> GAMGDVSRLNQRNINELKIFVEKAKYYSIKLDAIYNECTGAYNDIMTYSEGTFSDQSKVNQAISIFKKDNKIVNKFKELEKIIEEYKPMFLSKLIDDFAIELDQAVDNDVSNARHVADSYKKLRKSVVLAYIESFDVISSKFVDSKFVEASKKFVNKAKEFVEENDLIALECIVKTIGDMVNDREINSRSRANNFAKKEADFLGAAVELEGAYKAIKQTLL

Lyme borreliae produce other outer surface proteins, including CspZ (also known as BbCRASP-228,29). CspZ promotes bacterial dissemination to distal tissues by evading the complement system, the first-line innate immune defense in vertebrates in the blood, through binding and recruiting a host complement inhibitor, factor H (FH). Additionally, CspZ is only produced after Lyme borreliae invade vertebrate hosts and, as such, induces CspZ-specific immune responses after natural infection. Similar to CspZ, CspZ-YA is an all-α-helical protein composed of nine α-helices (denoted as helices A to I).

Here, we solve the crystal structure of a mutated Bb vaccine antigen, CspZ-YA that lacks the ability to bind to host complement factor H (FH). However, in CspZ-YA, the distance fluctuates between 2.6 and 31.8 Å but mostly greater than 4 Å. Such a distance is unfavorable for the formation of the salt bridge, suggesting the destabilization of CspZ-YA. Additionally, the three-dimensional structure of CspZ revealed a hydrophobic core between helices G, H and I where residues Y207 and Y211 are on one side, along with F176, I183 and F217 on the other side. Unlike CspZ, a cavity was found in CspZ-YA due to the replacement of two bulky and non-polar amino acid residues, Y207 and Y211, with alanine (the red highlight in Fig. 6D). Further, the altered conformation in CspZ-YA prevents R206 from interacting with E186, exacerbating the cavity-mediated structural instability. In Lyme borreliae CspZ proteins, the mutagenesis of Y207A and Y211A reduced the hydrophobic interactions and created a cavity at the C-terminal H/I loop and helix H of CspZ-YA, destabilizing the protein’s conformation. However, the RMSF values of R5 varied among these tested proteins with CspZ-YA having the highest flexibility (0.9–5.5 Å), followed by CspZ-YAC187S (0.9–5.0 Å), CspZ-YAI183Y (0.9–4.7 Å), and CspZ (0.9–2.2 Å).> SSKMDQLRPVLGRAGVDALWVSAPANVRWLSGFTSAEDGKVLVSPDGATLYTDARYTVQAQEESSLPQYIARPPATYEHAADTVRGLRVGFEAESLTVAELEDLRQAWPNSTLVALRGTLGGLRAVKTPEEIGAIRAAQDLADRVYTEVRPMIRAGVRELDVAVEIETRLRRAGGESAFELIVASGPNGAKPHGHASKRVIEDGDLVTIDMGARLGGYNS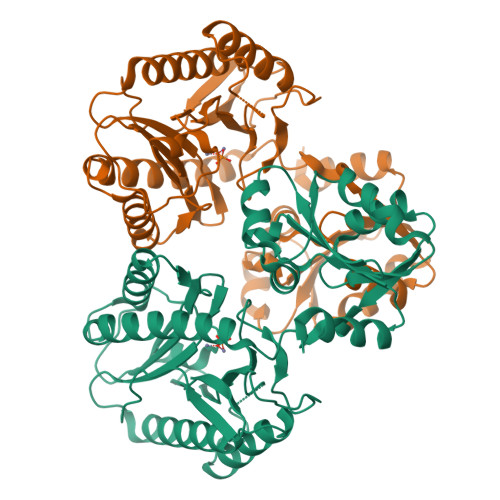DMTRTVAVGTPSAEMKRVYDAVLEAEEAAIAAIRPGVRAADLDKLARDLLTRHGLGEAFAHSLGHGVGLEVHEGPGLRGTSQDVLEAGMVITIEPGAYLPGVGGVRIEDLILVTEDGYEVLSHSAKESV>GSFDK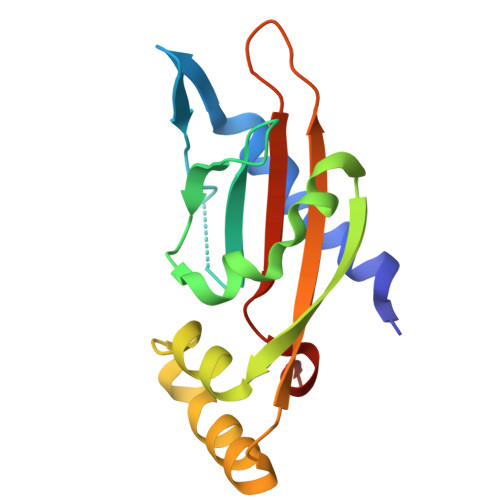TTFRLLRGESNLFYTLAKWENNKLHVELPENIDKQSPTMTLIYDENGQLLWAQRDVPWLMKMIQPDWLKSNGFHEIEADVNDTSLLLSGDHSIQQQLQEVREDDDDAEMTHSVAVNVYPATSRMPKLTIVVVDTIPVELKSSYM[2x]>[2x]MMISEDLRQKVLADAALGAGNVIHRLPLYGRSLDEEVLWLDGTWRAPDGSRPEVLTLGGLHEVVAEYAGFYTRAGVRAKDAVAIVSTSITDFALNLMALTGIGAIASLVNANMPAETRREYIRRQRV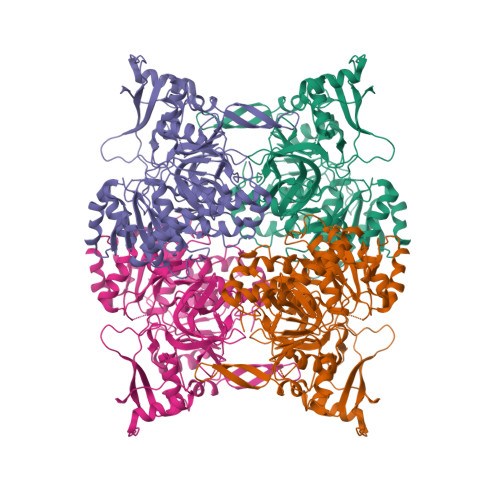VGIMTREPWHADLLAHLDDDEPPLFVALQSEVEPGNREHRPAAYPFRHAPGDPILISHSSGTTGIPKSAFHTHETLFHGALSRLADGLDCSTRKRLLALPGHHVSAMSNTLLGLTLGAPVVHYTDPSGKAVLDGIEKHRPTIVFGFTHTFTEMAAEDLTDRDLTSVEAYYASGDAAHAVHIRRLLDKGYHTATGPDLKPKKVPGAIFIDMFGSTEMGYVLFDFVHRAGGPVIGRCIGRPMRFAQAAVVGEDGSVLPPGQVGRLGVRSKSLTPGFWNDNVRWHKQWLGGYFLTGDLAYRDAANTFYHLDRTTDAIRTEEGFVYSAYTEEVLLREYPEILDCTVVGLADEGVEFGWEDEGVATVYALVNLVEGAEAPQDPTAWINEALGRAGLPRVAGAAIVTEDTIPVGITGKVLKRVVRAEARKLIGGCLEHHHHHHX The Nef protein of human (HIV) and simian (SIV) immunodeficiency viruses is an important replication and pathogenicity factor. Nef-mediated internalization of CD4 from the surface of infected cells is highly conserved among primate lentiviruses and thought to promote the release of fully infectious viral particles and to prevent superinfection. Nef stimulates clathrin-mediated endocytosis of CD3, CD4 and other cellular receptors by acting as an adapter of the adapter protein machinery. Our study thus provides insights into the molecular basis for the versatility of Nef as an adapter protein for the internalization of surface molecules containing endocytic sorting motifs.

The complex between SIVmac239 Nef 66–235 (SIV-B) and the SH3 domain of human Hck 80–140 (SH3E), engineered in the RT loop for improved Nef binding, yielded diffracting crystals. The structure was determined by molecular replacement at 2.78 Å resolution with good stereochemistry. The model contains residues 103–233 of SIV Nef and residues 80–134 of the SH3 domain, whereas no electron density was identified for the CD4 peptide. The asymmetric unit consists of two Nef/Hck heterodimers that assemble at the Nef–SH3 domain interface with the C-terminal flexible loop of Nef exposed in opposite directions. At the contact interfaces a three-fold rotational symmetry appears with each C-terminal flexible loop of Nef contacting the sorting motif recognition site of the neighboring Nef–SH3 heterodimer. In this crystallographic assembly, the EEHYLM sorting motif of the C-terminal flexible loop interacts with the hydrophobic crevice formed by the two central helices α4 and α5 of Nef and the interconnecting loop. As observed for HIV-1 Nef and its myristoylated full length variant, SIVmac239 Nef eluted as monomer in size exclusion chromatography experiments or as heterodimer in complex with the SH3 domain. Thus, the interaction of the ExxxLM sorting motif of one Nef molecule with the sorting motif recognition domain of another Nef molecule does not lead to multimerization in vitro.

>[2x]GAMATPWRNPAEEREKLAYRKQNMDDIDEEDDDLVGVSVRPKVPLRTMSYKLAIDMSHFIKEKGGLEGIYYSARRHRILDIYLEKEEGIIPDWQDYTSGPGIRYPKTFGWLWKLVPVNVSDEAQEDEEHYLMHPAQTSQWDDPWGEVLAWKFDPTLAYTYEAYVRYPEEFGS;>[2x]MEDIIVVALYDYEGWWGDLSFQKGDQMVVLEESGEWWKARSLATRKEGYIPSNYVARVDS>[2x]MATFQTDADFLLVGDDTS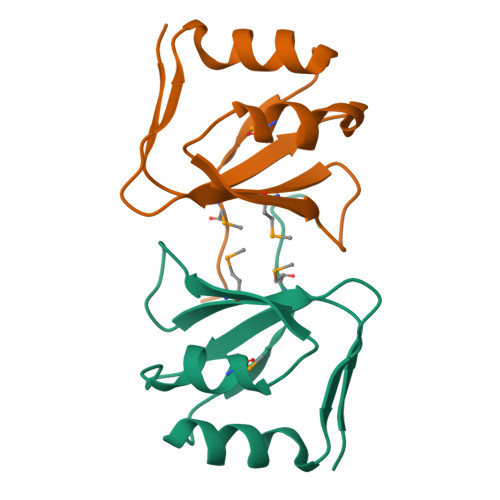RYEEVMKTFDTVEAVRKSDLDDRVYMVCLKQGSTFVLNGGIEELRLLTGDSTLEIQPMIVPTTELEHHHHHH>[4x]QFPRQCATVEALRSGMCCPDLSPVSGPGTDRCGSSSGRGRCEAVTADSRPHSPQYPHDGRDDREVWPLRFFNRTCHCNGNFSGHNCGTCRPGWRGAACDQRVLIVRRNLLDLSKEEK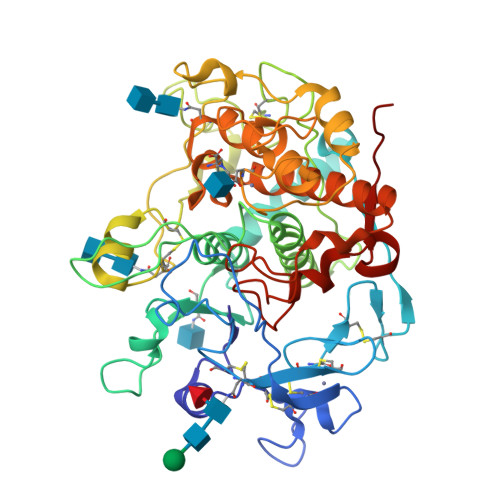NHFVRALDMAKRTTHPLFVIATRRSEEILGPDGNTPQFENISIYNYFVWTHYYSVKKTFLGVGQESFGEVDFSHEGPAFLTWHRYHLLRLEKDMQEMLQEPSFSLPYWNFATGKNVCDICTDDLMGSRSNFDSTLISPNSVFSQWRVVCDSLEDYDTLGTLCNSTEDGPIRRNPAGNVARPMVQRLPEPQDVAQCLEVGLFDTPPFYSNSTNSFRNTVEGYSDPTGKYDPAVRSLHNLAHLFLNGTGGQTHLSPNDPIFVLLHTFTDAVFDEWLRRYNADISTFPLENAPIGHNRQYNMVPFWPPVTNTEMFVTAPDNLGYTYEIQWPS> GSHMQCNVPLGMESGRIANEQISASSTYSDGRWTPQQSRLHGDDNGWRPNLDSNKEYLQVDLRFLTMLTAIATQGAISRETQNGYYVKSYKLEVSTNGEDWMVYRHGKNHKVFQANNDATEVVLNKLHAPLLTRFVRIRPQTWHSGIALRLELFGCRVTDAPCSNMLGMLSGLIADSQISASSTQEYLWSPSAARLVSSRSGWFPRIPQAQPGEEWLQVDLGTPKTVKGVIIQGARGGDSITAVEARAFVRKFKVSYSLNGKDWEYIQDPRTQQPKLFEGNMHYDTPDIRRFDPIP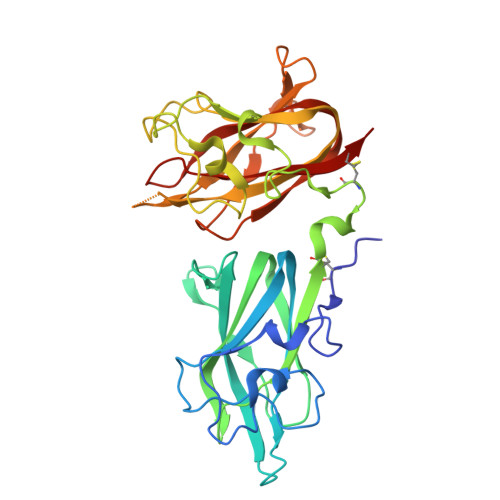AQYVRVYPERWSPAGIGMRLEVLGCDWT(4-methyl-1,3-thiazol-5-yl)methyl 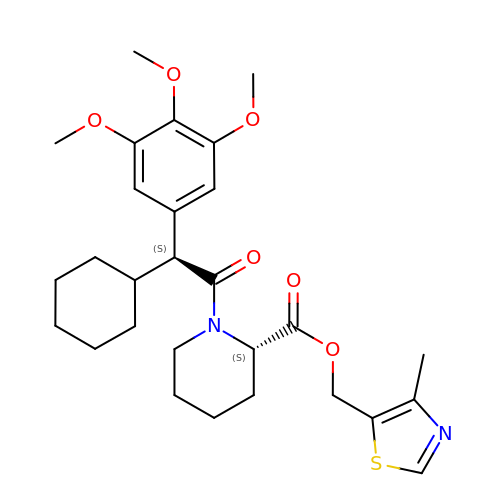(2S)-1-[(2S)-2-cyclohexyl-2-(3,4,5-trimethoxyphenyl)ethanoyl]piperidine-2-carboxylate | C28 H38 N2 O6 S | QGFACBYRMIEZCB-OFVILXPXSA-N> MSRSKRDNNFYSVEIGDSTFTVLKRYQNLKPIGSGAQGIVCAAYDAILERNVAIKKLSRPFQNQTHAKRAYRELVLMKVVNHKNIIGLLNVFTPQKSLEEFQDVYIVMELMDANLSQVIQMELDHERMSYLLYQMLVGIKHLHSAGIIHRDLKPSNIVVKSDATLKILDFGLARTAGTSFMMTPYVVTRYYRAPEVILGMGYKENVDIWSVGCIMGEMIKGGVLFPGTDHIDQWNKVIEQLGTPSPEFMKKLQPTVRTYVENRPKYAGYSFEKLFPDVLFPADSEHNKLKASQARDLLSKMLVIDASKRISVDEAL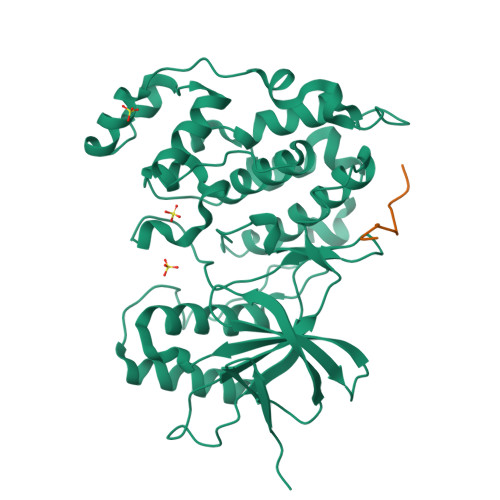QHPYINVWYDPSEAEAPPPKIPDKQLDEREHTIEEWKELIYKEVMDLEHHHHHH;> RPKRPTTLNLF>[5x]SKGLEDSSTISFI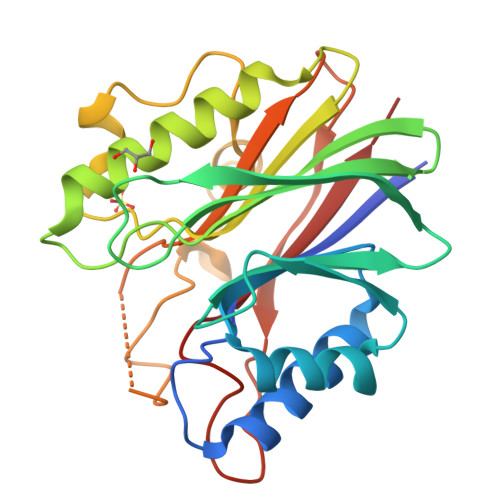TWNIDGLDGCNLPERARGVCSCLALYSPDVVFLQEVIPPYCAYLKKRAASYTIITGNEEGYFTAILLKKGRVKFKSQEIIPFPNTKMMRNLLCVNVSLGGNEFCLMTSHLESTREHSAERIRQLKTVLGKMQEAPDSTTVIFAGDTNLRDQEVIKCGGLPDNVFDAWEFLGKPKHCQYTWDTKANNNLRIPAAYKHRFDRIFFRAEEGHLIPQSLDLVGLEKLDCGRFPSNHWGLLCTLNVVL RlmCD is a recently identified MTase for ribosomal RNA in S. pneumoniae. Similar to its homologue YefA in B. subtilis, RlmCD can catalyze m5U methylation for both U747 and U1939 of 23S rRNA, whereas these two modifications are catalyzed by two different enzymes RlmC and RumA, respectively, in E. coli. Our structural evidences indicate that RlmCD is a MTase that belongs to the RFM family. All together, our in-vitro experiments confirmed that RlmCD is a 23S rRNA MTase specific for U747.

To learn the structural basis for RlmCD-substrate binding specificity, we co-crystalized RlmCDs with SAM and 18-mer U747-methylated rRNA helix 35 in S. pneumoniae (5’-740GGCACGUm5UGAAAAGUGCC757-3’). In order to trap the complex in an inactive state favorable for crystallization, E443 in RlmCDs was mutated to glutamine (E443Q) as described in previous research. The crystal structure of the ternary complex was finally determined at 2.85Å with Rwork and Rfree values of 20% and 24%. Different from the apo-form structure, each asymmetric unit of the ligand-bound form contains four molecules (protomers A-D) of the complex, in which the electron densities of SAH molecules, rather than SAM, in protomers A and C were well-defined while those in protomers B and D were partially observed. The cofactor in the complex structure was therefore identified as SAH, even though SAM was used for crystallization. On the other hand, the electron density of the RNA molecule can only be observed in one complex per asymmetric unit. A double-helical RNA representing the five base-pairs in the stem region of helix 35 can be fitted into this density whereas the loop region cannot be modeled due to the lack of the extra electron density. In its complex structure, the SAH molecule is enveloped in a deep pocket on the surface of the C-terminal MTase domain while the same pocket is also utilized to accommodate SAH in RumA. The adenine ring and ribose of SAH lay down in the shallow area while the homocysteine part is entirely buried into the adjacent acidic pocket mainly constituted by the residues from α6 and α7, and the residues of the linker connecting α6 and β14. In our complex structure, although the quality of the electron-density map corresponding to the RNA is low, a double-helical RNA representing the five base-pairs in the stem region of helix 35 can be fitted without too much difficulty but the loop region including U747 can’t be modeled due to absence of excessive electron density. This double-helical RNA binds the cleft between the N-terminal TRAM and the catalytic domains of RlmCD in a similar mode as in RumA-RNA complex structure.

>MLKKNDIVEVEIVDLTHEGAGVAKVDGLVFFVENALPSEKILMRVLKVNKKIGFGKVEKYLVQSPHRNQDLDLAYLRSGIADLGHLSYPEQLKFKTKQVKDSLYKIAGIADVEVAETLGMEHPVKYRNKAQVPVRRVNGVLETGFFRKNSHNLMPLEDFFIQDPVIDQVVVALRDLLRRFDLKPYDEKEQSGLIRNLVVRRGHYSGQIMVVLVTTRPKVFRVDQLIEQVIKQFPEIVSVMQNINDQNTNAIFGKEWRTLYGQDYITDQMLGNDFQIAGPAFYQVNTEMAEKLYQTAIDFAELKKDDVIIDAYSGIGTIGLSVAKHVKEVYGVELIPEAVENSQKNASLNKITNAHYVCDTAENAMKKWLKEGIQPTVILVDPPRKGLTESFIKASAQTGADRIAYISCNVATMARDIKLYQELGYELKKVQPVDLFPQTHHVQTVALLSKLDVD[4x]~{N}-[2-(1~{H}-pyrrolo[2,3-b]pyridin-5-yl)phenyl]propanamide | C16 H15 N3 O | 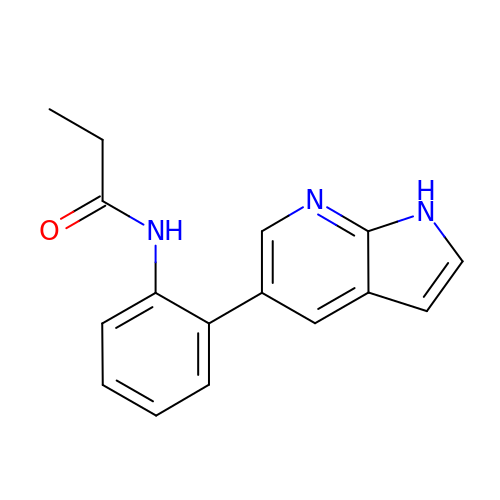ZSLQYIORPJSVTD-UHFFFAOYSA-N> MTIDEIIEAIEKLTVSELAELVKKLE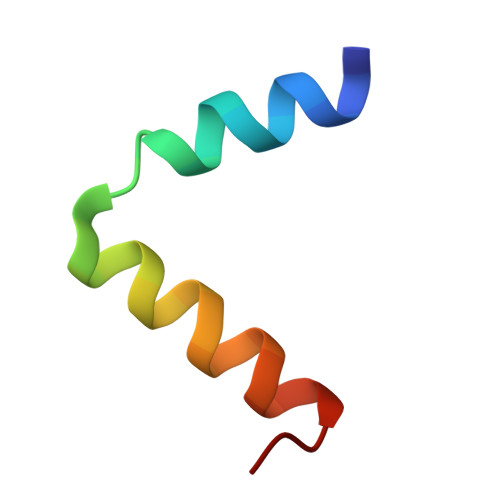DKFGVT In sequence analysis, enzyme EstDL136 was found to be a member of the HSL family. EstDL136 exhibits two different activities for the catalytic metabolism of chloramphenicol (Cm), a widely used, broad-spectrum antibiotic; it acts as both a Cm acetate esterase (CAE) and a Cm hydrolase. EstDL136 cleaves the amide linkage at C2 of Cm and thereby confers Cm resistance to bacteria heterologously expressing the EstDL136 gene. Structural analyses in this study have validated that EstDL136 contains structural features characteristic of the HSL family, with an α/β hydrolase fold and a CAP domain.

A crystal of EstDL136(ΔPMP) contains two monomers per asymmetric unit. Monomeric EstDL136(ΔPMP) consists of an N-terminal CAP domain and an α/β hydrolase domain. In addition to the core α/β fold, the 40-residue segment at the N-terminus forms a helix-loop-helix arrangement known as a CAP domain, in which α1 is almost orthogonal to α2 and protrudes from the main α/β fold. The putative catalytic triad, Asp252-His282-Ser156, is located at the C-terminal end of the central β-strands. EstDL136 has a relatively shallow, pocket-shaped active site, consistent with its substrate preference for p-nitrophenyl acetate over p-nitrophenyl butyrate. Residues Trp86, Met211, and Trp215 are clustered at the bottom of the active site in EstDL136(ΔPMP) and possibly occlude the active site pocket. Two monomers in an asymmetric unit show a non-crystallographic, two-fold symmetry. Interestingly, the CAP domains of the two monomers are in a domain-swap configuration in which the N-terminal helix α1 of the CAP domain almost intercalates into the potential vacancy between α1* and the main α/β fold of the adjacent monomer. As a result, the N-terminal helices α1 and α1* are packed in an anti-parallel orientation in the dimer. Under these structural conditions, it is unlikely that the dimer observed in crystalline EstDL136(ΔPMP) represents a biologically relevant oligomeric conformation, but its structural features could still provide details on the monomeric enzyme with the active site residues.

>[2x]MPLNPHVEALLQMMAQMPAPDFSVANPAEIRAVFDNLAAPPQVARVENIAISLDGRDLDARLYVPEDADERPALMVYYHGGGWVIGTLDTHDGTCRALAQKSGCAVLSIAYRLAPEYRYPAPAEDCYDALVWAKQNAATLGVDGDRLAVGGDSAGGNLAAAVAIMARDRNGPALRHQLLIYPVTDNDFTLASYAENGGGEYYLSTDGMRWFWGHYLGDTAAENAPLAAVLNVADLSGLAPATVITAEYDPLRDEGIAYAKKLDAAGVPVDAATAPGMIHGFFSMFEAVPDSWEWIERGASNLKRDLALEHHHHHHHH> GSPEKILAQIIQEHREGLDWQEAATRASLSLEETRKLLQSMAAAGQVTLLRVENDLYAISTERYQAWWQAVTRALEEFHSRYPLRPGLAREELRSRYFSRLPARVYQALLEEWSREGRLQLAANTVALAGFTPSFSETQKKLLKDLEDKYRVSRWQPPSFKEVAGSFNLDPSELEELLHYLVREGVLVKINDEFYWHRQALGEAREVIKNLASTGPFGLAEARDALGSSRKYVLPLLEYLDQVKFTRRVG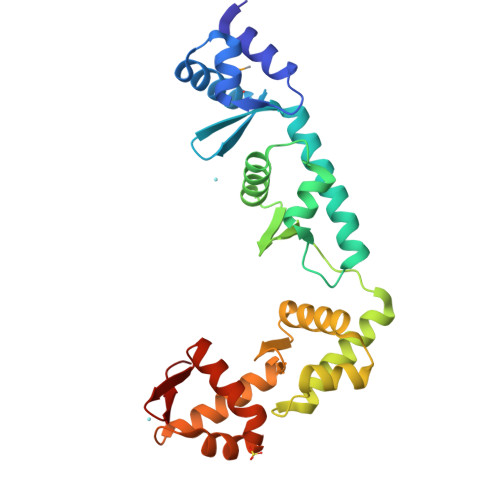DKRVVVGN>MRLRHENKIYKLM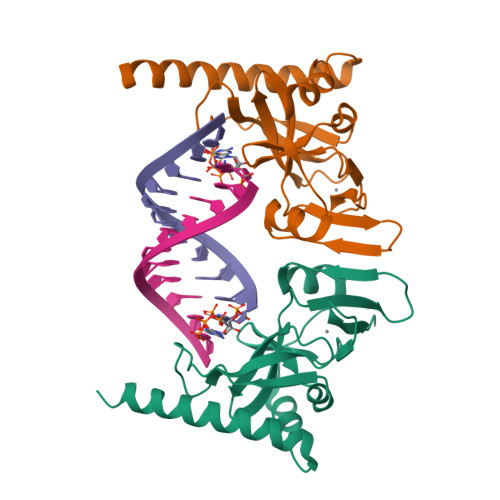CSNCSKEFCKSIYIKKVFSNYMVFDPSVWRFLHVESKRKVSKYLSEDNQPLSDIKCFHCKLDVGRAYKIRGTYLPQLSVKALTFVQESDYSSMTKAKWSDVEQDLFYISEAIEDDFRIMLNALSDTEENIEKKIVLDLDSRQHNKQLEMKRFHIQQE[2x]>[6x]MFSPSTTTLFRFVECTED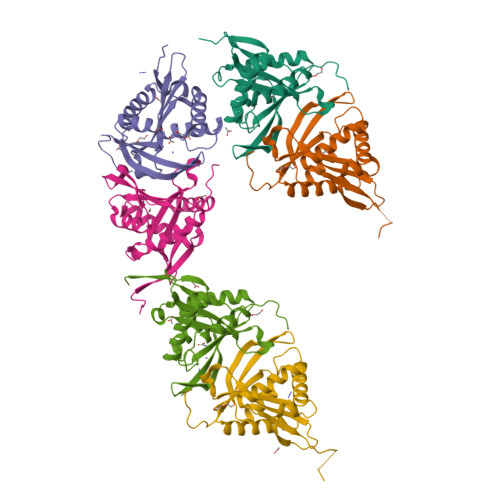QHALEILEILNDAIINSTALYDYKPRSKESMAAWFATKRQNNFPIIGAVNEVGQLLGFASWGSFRAFPAYKYTVEHSVYIHKDYRGLGLSKHLMNELIKRAVESEVHVMVGCIDATNVASIQLHQKLGFIHSGTIQQAGFKFGRWLDAAFYQLTLDTPLHPQDD> ADIGSTNDALDYYLKSKGFNGLFSQIELSFSASNLRDRDVLSKSDPMVVVYQKEKDATLSEVFRSEVVLNSLAPKWIKKFIVAYHFETVQTLVFRVYDVDTKFQNSREEMLKLDEQQFLGEATCALSEIITKSTRTSTLELKRKDGFAPQAQPHHGKLIIHAEESLASKISTEIVFRCSNLESKDLFSKSDPFLVVSKIVEHGTPIPVSKTEVRKNDLNPIWKPVFLSVQQVGSKDSPVIIECSDFNSNGKHSLIGKVQKSLSDLEKLHLAGQGINFSLPTGAGQNKVLKSQLFVDKFTETVHHTFLEYLASGFELNFMVAIDFTASNGNPRLPDSLHYIDPSGRLNAYQRAIMDVGEVLQFYDSDKRFPAWGFGARPIDAPVSHCFNL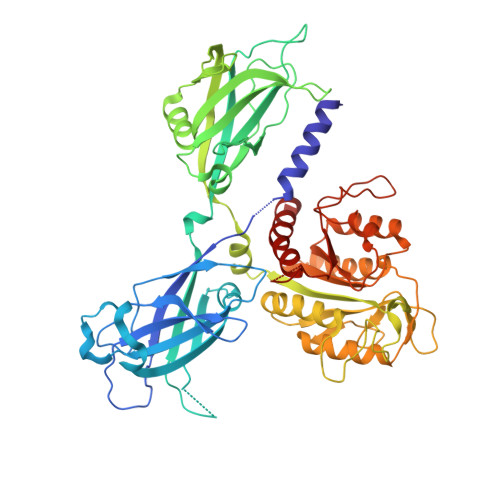NGSSSYSEVDGIQGIMTSYTSALFNVSLAGPTLFGPVINAAAMIASASLAQGSRKYYVLLIITDGVITDLQETKDALVSASDLPLSILIVGVGGADFKEMEILDADKGERLESSSGRLASRDIVQFVALRDVQYGEISVVQALLAELPSQFLTYMRIRN>[6x]AIATYNSHVELAKYLVSKADSVYLTIGKSTPWSNETNPPQPDENATVLQEVIGYKKATKVTLVRPSKSPEDDNKNLISYGN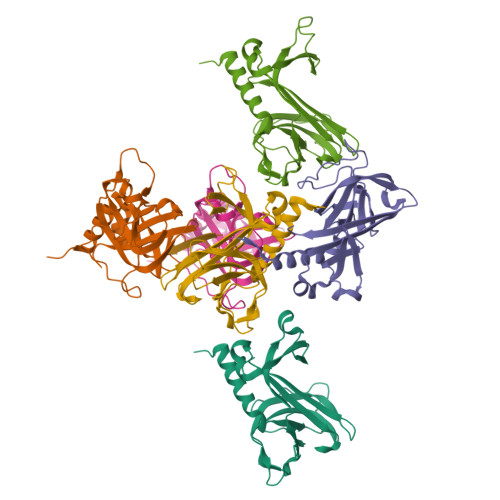KSWVEVTPENAKAEGAKWVYLESSIVGDELPLGTYRQVGFVMDLVAKSGISKFNLVPSEVESTGTLLFFDNKQFQNRSEQTTAKERFIVEVDP>[2x]MGSSHHHHHHSGLVPRGSHMATPPKRSSPSFSASSEGTRIKKISIEGNIAAGKSTFVNILKQLSEDWEVVPEPVARWSNVQSTQDEFEELTMSQKNGGNVLQMMYEKPERWSFTFQTYACLSRIRAQLASLNGKLKDAEKPVLFFER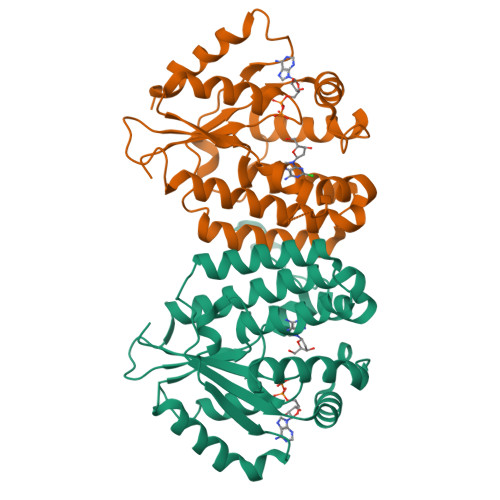SVYSDRYIFASNLYESESMNETEWTIYQDWHDWMNNQFGQSLELDGIIYLQATPETCLHRIYLRGRNEEQGIPLEYLEKLHYKHESWLLHRTLKTNFDYLQEVPILTLDVNEDFKDKYASLVEKVKEFLSTL>[6x]GAMAIPKIASYSIPLAETFPKNKVHWHV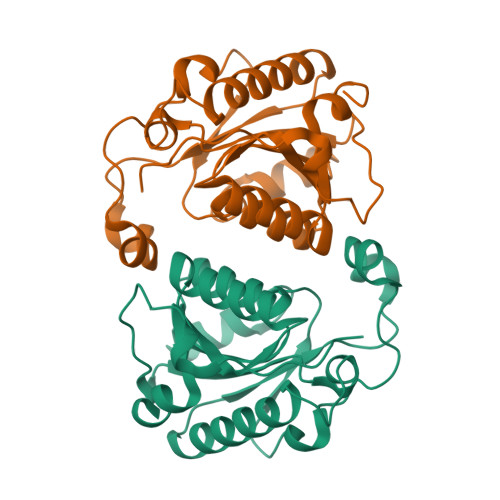QADRAVLLIHDMQKYFINFFDHSQAPVPELLANISELKSLARQANIPVVYTAQPPNQDPIERALLTDFWGTGLTKDTEIVSELSPEDGDIQYTKWRYSAFKKTPLLERMKETQRDQLIIVGVYAHIGILSTALDAFMLDIQPFVVGDAVADFSLEDHHHTLKYITERVGCVTSLEALKPQMIHSQETRLLS>MDSLQKQDLRRPKIHGAVQASPYQPPTLASLQRLLWVRQAATLNHIDEVWPSLFLGDAYAARDKSKLIQLGITHVVNAAAGKFQVDTGAKFYRGMSLEYYGIEADDNPFFDLSVYFLPVARYIRAALSVPQGRVLVHCAMGVSRSATLVLAFLMIYENMTLVEAIQ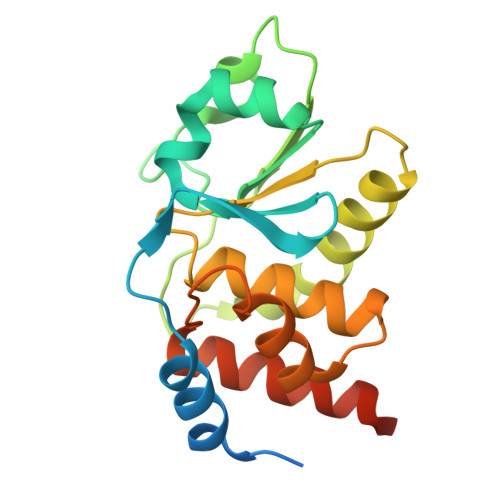TVQAHRNICPNSGFLRQLQVLDNRLGRETGRFAHHHHHH[4x]> PISADFSEVENAPSFLSLAENTDEVLKPYTGLEIQTIITNIVGDANPNQSRIFDQDRLRGNQYSAGGLVTQNAVSAIPFTNLIPRTIRVGNILVNSANRLQITETNVSEYYSNPIIATKLSEMISDQVKNNQFSTWRRDNTSLQGFNAFDIATINTAILPNGLSLESMLLKLSLLHSIKAMNVDAASINRSQYQVIDHNTVPTIGAPAVVGVNNSPVFGEDCGGNNPVYPFGGGTGAIAFHVTLQTVPDERKSYAIFVPPAILQATSDANEALALFALSMSEWPHALYTVTKQTTDLAGANAGQQVFIPTQSTIHIGGRRVLDLIIPRREIAPNPTTLVAANAMCMVRPQAGPDATAGAIPLAAGQLFNMNFIGAPAFEEWPLTSYLYSWAGRFDITTIRQYMGRLATMVGVKDAYWAAHELNVALSQVAPKMTTAAGGWAAQAANSAQQSDVCYSSLLTVTRSAANFPLANQPAADMRVYDTDPATWNKVALGLATAANLVPEQSMDVPFVVGDARTSFWERLQAIPMCIAWTMYYHSRGI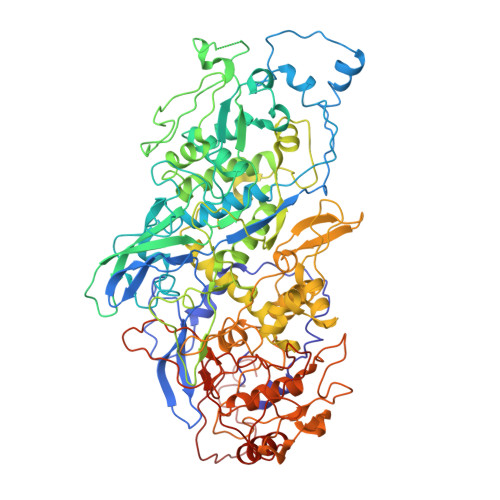TTLAWDNAYTDNTNKWLQKMVRNTFSTTQSVGTIIPARYGKIVCNLYKNMFHRAPAYVATSVGGKELHITHFERWLPGGTYANVYSGAGAVVNCFSPVLIPDIWCQYFTAKLPLFAGAFPPAQGQNSTKGFNSKQGLMIHRNQNNNLVAPYLEKFADNSSYFPVGQGPEINDMATWNGRLWMTTGNVQYLDYSGAAIVEAVPPAGELPVGKQIPLLAGENAPIELTNAATTCVPRYSNDGRRIFTYLTTAQSVIPVQACNRAANLARSCWLLSNVYAEPALQALGDEVEDAFDTLTNS>SLWQPQTGDIIFQISRSSQSKAIQLATHSDYSHTGMLVMRNKKPYVFEAVGPVKYTPLKQWIAHGEKGKYVVRRVEGGLSVEQQQKLAQTAKRYLGKPYDFSFSWSDDRQYCSEVVWKVYQNALGMRVGEQQKLKEFDLSNPLVQAKLKERYGKNIPLEETVVSPQAVFDAPQLTTV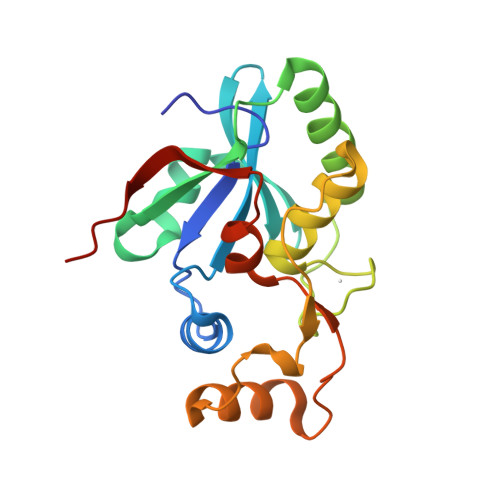AKEWPLFSW[2x]>[2x]GAMGSGIQRPTSTMTTSLDKQLWELIDNFFLKAALLICHSKGWKGAPAADEGPPTTNSWFNIETFGDTKLERELKPWTTFDGSESLPPLVIETYLDLARLSPSQQVTLKDQDGNPWNVCKGTKKSEIMLERWLIQMDNGEDSPSLQSSGSEDTDDNVSELYRQLVLLFRYLETLVGLLPASELQARLIRPGVSPEAPPPVKLGTRILDGSKPIVSKG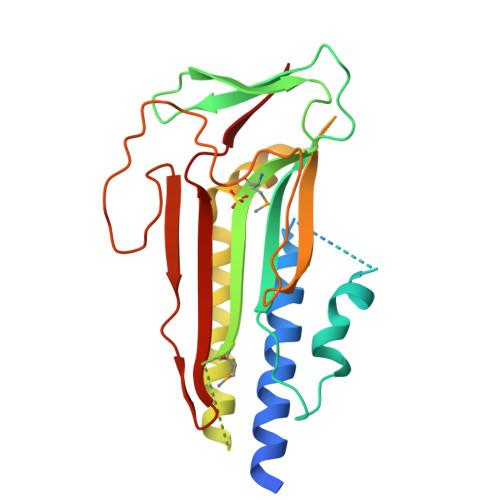RIGLSKSLIATYSNVINETNLPAHLEQRKITPIRTKFGSLRISVSYRKDCDFHVNG>[2x]TVAYIA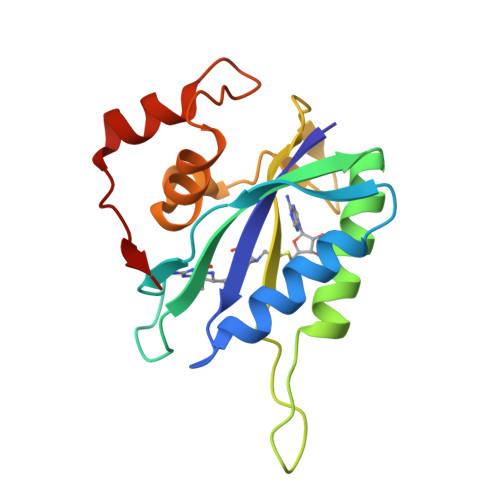IGSNLASPLEQVNAALKALGDIPESHILTVSSFYRTPPLGPQDQPDYLNAAVALETSLAPEELLNHTQRIELQQGRVRKAERWGPRTLDLDIMLFGNEVINTERLTVPHYDMKNRGFMLWPLFEIAPELVFPDGEMLRQILHTRAFDKLNKW>GSAKDPMQIGNFNTDKKVFIIAELSANHAGSLEMALKSIKAAKKAGADAIKIQTYTPDSLTLNSDKEDFIIKGGLWDKRKLYELYESAKTPYEWHSQIFETAQNEGILCFSSPFAKEDVEFLKRFDPIAYKIASFEANDENFVRLIAKEKKPTIVSTGIATEEELFKICEIFKEEKNPDLIFLKCTSAYPAAIEDMNLKGIVSLKEKFNVEVGLSDHSFGFLAPVMAVALGARVIEKHFMLDKSIESEDSKFSLDFDEFKAMVDAVRQAESALGDDKLDLDEKALKNRVFARSLYASKDIKKGEIFSE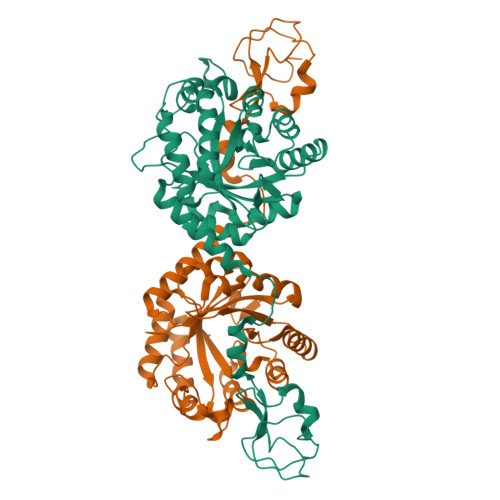ENVKSVRPSFGLHPKFYQELLGKKATKDIKFGDALKQGDFQ[4x]> SAKDERAREILRGFKLNWMNLRDAETGKILWQGTEDLSVPGVEHEARVPKKILKCKAVSRELNFSSTEQMEKFRLEQKVYFKGQCLEEWFFEFGFVIPNSTNTWQSLIEAAPESQMMPASVLTGNVII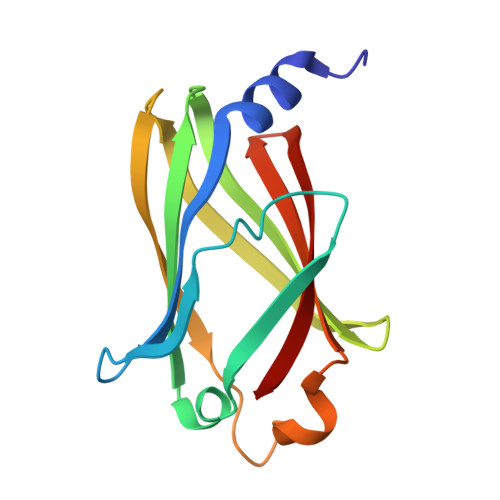ETKFFDDDLLVSTSRVRLFYV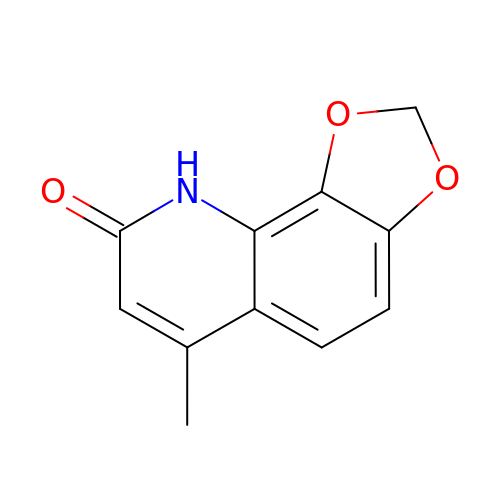6-methyl[1,3]dioxolo[4,5-h]quinolin-8(9H)-one | C11 H9 N O3 | XCKXJOHJSMHNFE-UHFFFAOYSA-N> DNGGYVPAVVIGTGYGAAVSALRLGE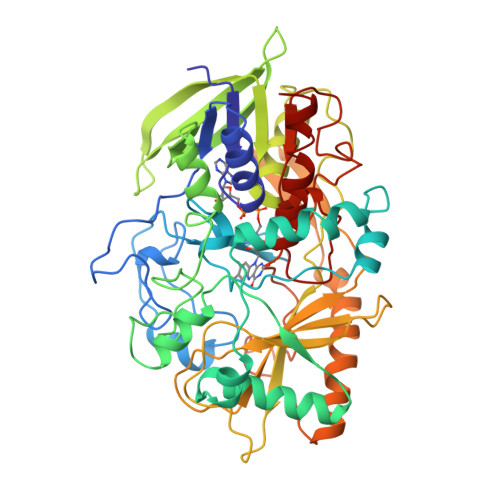AGVQTLMLEMGQLWNQPGPDGNIFCGMLNPDKRSSWFKNRTEAPLGSFLWLDVVNRNIDPYAGVLDRVNYDQMSVYVGRGVGGGSLVNGGMAVEPKRSYFEEILPRVDSSEMYDRYFPRANSMLRVNHIDTKWFEDTEWYKFARVSREQAGKAGLGTVFVPNVYDFGYMQREAAGEVPKSALATEVIYGNNHGKQSLDKTYLAAALGTGKVTIQTLHQVKTIRQTKDGGYALTVEQKDTDGKLLATKEISCRYLFLGAGSLGSTELLVRARDTGTLPNLNSEVGAGWGPNGNIMTARANHMWNPTGAHQSSIPALGIDAWDNSDSSVFAEIAPMPAGLETWVSLYLAITKNPQRGTFVYDAATDRAKLNWTRDQNAPAVNAAKALFDRINKANGTIYRYDLFGTQLKAFADDFCYQPLGGCVLGKATDDYGRVAGYKNLYVTDGSLIPGSVGVNPFVTITALAERNVERIIKQDVTAS> SHSGFKCPICSKSVASDEMEMHFIMCLSKPRLSYNDDVLTKDAGECVICLEELLQGDTIAR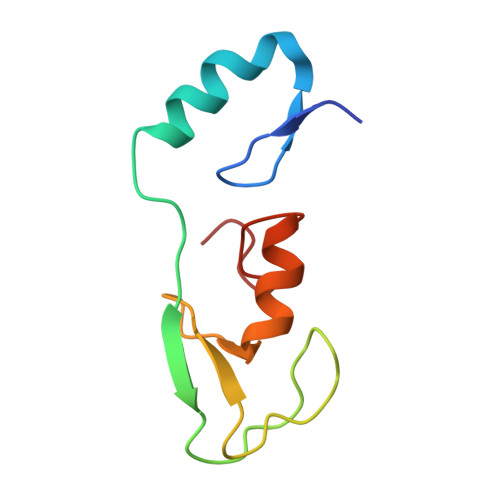LPCLCIYHKSCIDSWFEVNRSCPEHPAD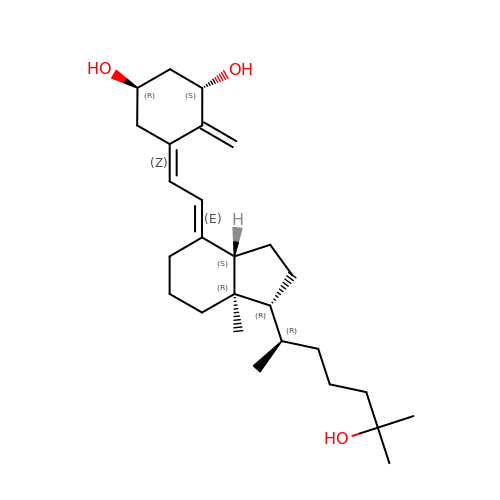5-{2-[1-(5-HYDROXY-1,5-DIMETHYL-HEXYL)-7A-METHYL-OCTAHYDRO-INDEN-4-YLIDENE]-ETHYLIDENE}-4-METHYLENE-CYCLOHEXANE-1,3-DIOL | C27 H44 O3 | GMRQFYUYWCNGIN-NKMMMXOESA-N>[2x]MNSSLPSLRDVFANDFRIGAAVNPVTIEMQKQLLIDHVNSITAENHMKFEHLQPEEGKFTFQEADRIVDFACSHRMAVRGHTLVWHNQTPDWVFQDGQGHFVSRDVLLERMKCHISTVVRRYKGKIYCWDVINEAVADEGNELLRPSKWRQIIGDDFMEQAFLYAYEADPDALLFYNDYNECFPEKREKIFALV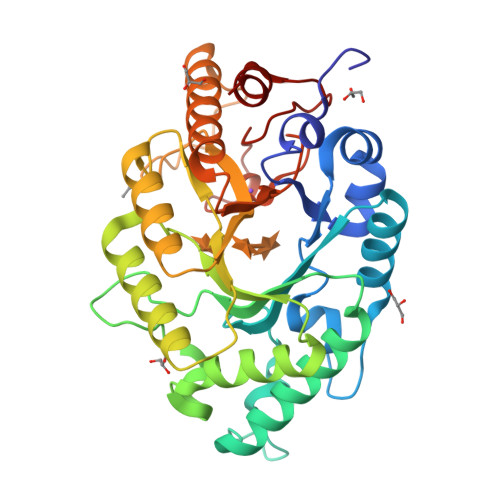KSLRDKGIPIHGIGMQAHWSLTRPSLDEIRAAIERYASLGVVLHITELDVSMFEFHDRRTDLAAPTSEMIERQAERYGQIFALFKEYRDVIQSVTFWGIADDHTWLDNFPVHGRKNWPLLFDEQHKPKPAFWRAVSV>MAEIGTGFPFDPHYVEVLGERMHYVDVGPRDGTPVLFLHGNPTSSYVWRNIIPHVAPTHRCIAPDLIGMG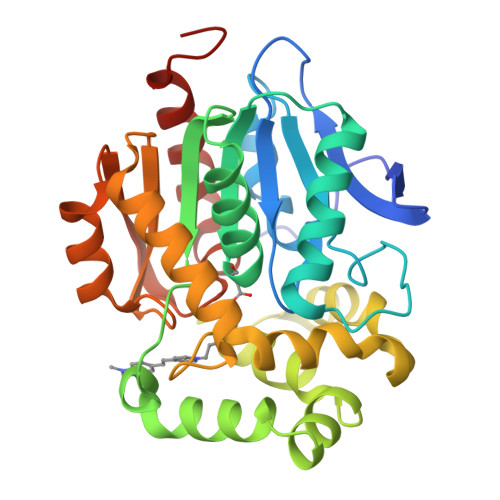KSDKPDLGYFFDDHVRFMDAFIEALGLEEVVLVIHDWGSALGFHWAKRNPERVKGIAFMEFICPIPTWDEWPMHARETFQAFRTTDVGRKLIIDQNVFIEGTLPYGVVRPLTEVEMDHYREPFLNPVDREPLWRFPNELPIAGEPANIVALVEEYMDWLHQSPVPKLLFWGTPGALIPPAEAARLAKSLPNCKAVDIGPGLNLLQEDNPDLIGSEIARWLSTLEISGHHHHHH[2x]>MKVLSYLKNFYLFLAIGAIMQASE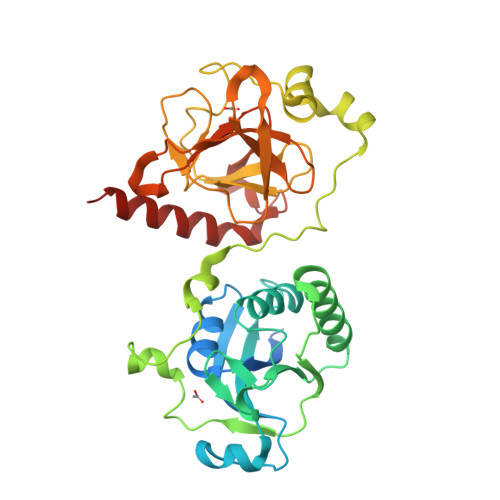NMGSQHQKTDERVIYLAGGSFWGLEAYMERIYGVIDASSGYANGKTSSTNYEKLHESDHAESVKVIYDPKKISLDKLLRYYFKVVDPVSVNKQGNDVGRQYRTGIYYVNSADKEVIDHALKALQKEVKGKIAIEVEPLKNYVRAEEYHQDYLKKHPSGYCHIDLKKADEVIVDDDKYTKPSDEVLKKKLTKLQYEVTQNKHTEKPFENEYYNKEEEGIYVDITTGEPLFSSADKYDSGCGWPSFSKPINKDVVKYEDDESLNRKRIEVLSRIGKAHLGHVFNDGPKELGGLRYSINSAALRFIPLKDMEKEGYGEFIPYIKKGELKKYINDKKSH[2x]>MGSSHHHHHHENLYFQGSMNISVFDLFSIGIGPSSSHTVGPMLAANAFLQLLEQKNLFDKTQRVKVELYGSLALTGKGHGTDKAILNGLENKAPETVDPASMIPRMHEILDSNLLNLAGKKEIPFHEATDFLFLQKELLPKHSNGMRFSAFDGNANLLIEQVYYSIGGGFITTEEDFDKSTTDTNPPPYPFATATELLKLCKKHHLTIAELMLVNEKTWRSTAEIHKGILDIAKVMDDCINNGCKHDGVLPGGLNLKRRAPDLYRKLIEQKGVKSVFEQSDIMNHLNLYAMAVNEENAAGGRIVTA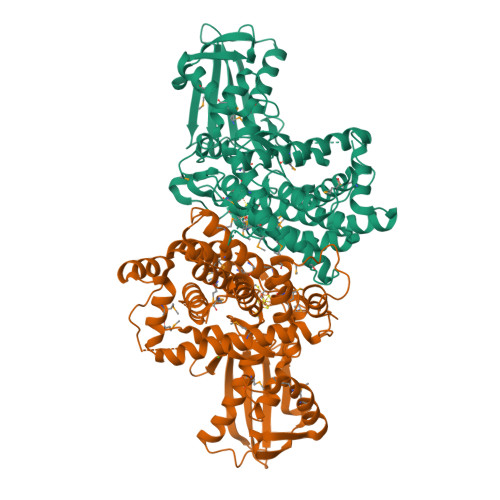PTNGAAGIIPAVLKYCQQAHDRMSNEDIYTYFLTAAAIGILYKKGASISGAEVGCQGEVGVASSMAAAGLTAVLGGTIEQVENAAEIAMEHHLGMTCDPVLGLVQIPCIERNAMGAVKAVNATRMALIGDGQHQISLDKVIKTMKQTGMDMQSIYKETSMGGLAVNLPEC[2x]>ALYEDPPDQKTSPSGKPATLKICSWNVDGLRAWIKKKGLDWVKEEAPDILCLQQTKCSENKLPAELQELPGLSHQYWSAPSDKEGYSGVGLLSRQAPLKVSYGIGDEEHDQEGRVIVAEFDSFVLVTAYVPNAGRGLVRLEYRQRWDEAFRKFLKGLASRKPLVLCGNLNVAHEEIDLRNPKGNKKNAGFTPQERQGFGELLQAVPLADSFRHLYPNTPYAYT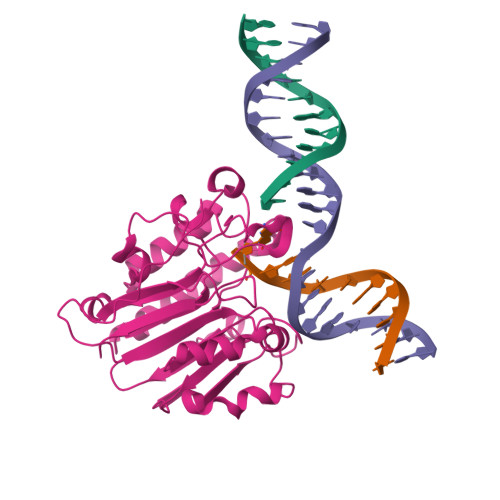FWTYMMNARSKNVGWRLDYFLLSHSLLPALCDSKIRSKALGSDHCPITLYLAL[2x]>[4x]MGSDKIHHHHHHENLYFQGMLYDLTVVQFSKMLKNLNAIFDKAEAFAELKKVDMDVLLNSRLAADQFNLIRQVQ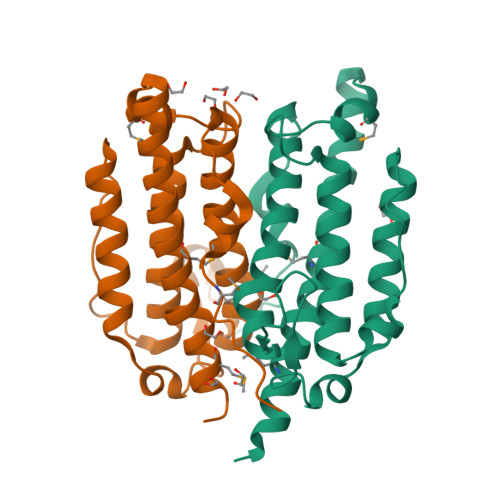IACDTAKVGVARLTGQLETAPKHDDSETTLAELRQRIASVLTYLEGFSEADFANAATIQISQPRWQGKYLTGYEFAIEHAIPNLYFHITTAYGILRHNGVEVGKKDYLGAMPYKAPIL> MALALLEDWCRIMSVDEQKSLMVTGIPADFEEAEIQEVLQETLKSLGRYRLLGKIFRKQENANAVLLELLEDTDVSAIPSEVQGKGGVWKVIFKTPNQDTEFLERLNLFLEKEGQTVSGMFRALGQEGVSPATVPCISPELLAHLLGQAMAHAPQPLLPMRYRKLRVFSGSAVPAPEEESFEVWLEQATEIVKEWPVTEAEKKRWLAESLRGPALDLMHIVQADNPSISVEECLEAFKQVFGSLESRRTAQVRYLKT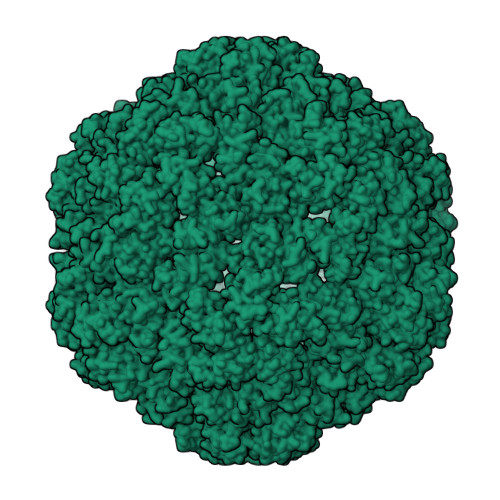YQEEGEKVSAYVLRLETLLRRAVEKRAIPRRIADQVRLEQVMAGATLNQMLWCRLRELKDQGPPPSFLELMKVIREEEEEEASFENESIEEPEERDGYGRWNHEGDD>APQQINDIVHRTITPLIEQ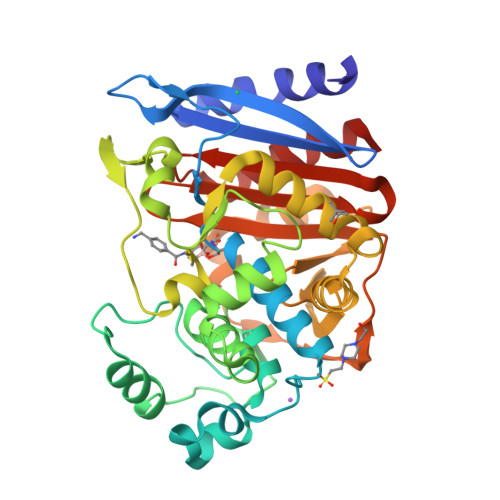QKIPGMAVAVIYQGKPYYFTWGYADIAKKQPVTQQTLFELGSVSKTFTGVLGGDAIARGEIKLSDPTTKYWPELTAKQWNGITLLHLATYTAGGLPLQVPDEVKSSSDLLRFYQNWQPAWAPGTQRLYANSSIGLFGALAVKPSGLSFEQAMQTRVFQPLKLNHTWINVPPAEEKNYAWGYREGKAVHVSPGALDAEAYGVKSTIEDMARWVQSNLKPLDINEKTLQQGIQLAQSRYWQTGDMYQGLGWEMLDWPVNPDSIINGSDNKIALAARPVKAITPPTPAVRASWVHKTGATGGFGSYVAFIPEKELGIVMLANKNYPNPARVDAAWQILNALQ[4x]> HHHHHHGSATIDGIIQGSVHSALTGESYGESVKQAVILNVVGGGDSIADPLSPGENDMVHRLKRLEDEQKGEIIRTKHNAQVIAKFGRDLEDVYKFASREHKVGEEEEDQIQMLEKALRAYGNVVKVEGESVQKLAKALRAEEEERTDEETRMIGEYRDKIDALSKAIEIEREGLQDEAIQEIAGMSAEVLEAAAEEVPIFGAGVATSIATARAIEGAYKLKAVITALTGIDLSHMTTPKIQPKTLEAILDAPGGNVTDLMLTRGLDSKIDKINENLAEVEHMQTSILPRIKKAIEEDRDEITNWSPKRIHPKSVQRFRVPRMQTPSIHIYAAPWDSDSVFIFHVISPHHLNESFFLGFDLEIEYVHYEDLAQHWHSLGAAQEVTGRTFREAYREFFNLASRSTM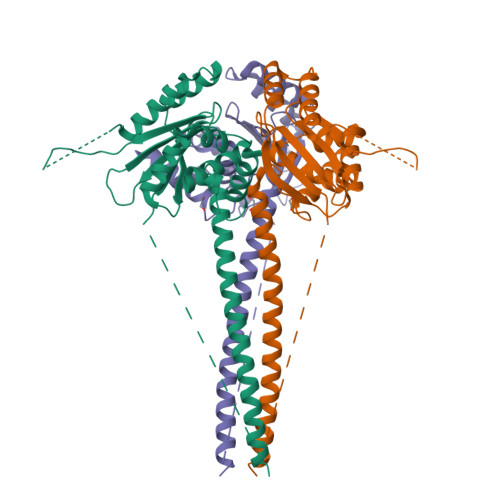ASDIHKKRLQRSRMSHPIYLGVHNYELSYIAIKSNAMQLVTDEDLQKHVLRGPLHFQRRVIMAALKYGVKVMSRADDIAMMLRDA>[4x]SNAMSEWSRI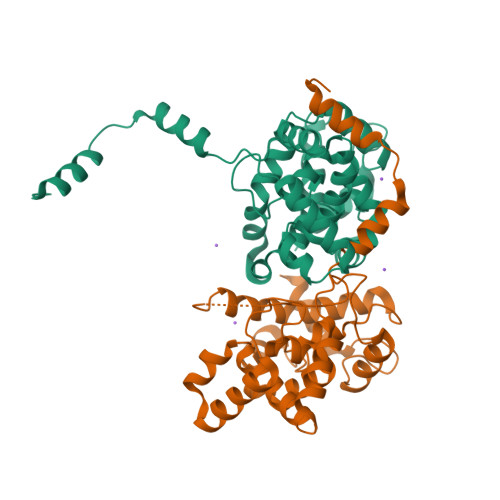AVEFGEQQLNLTELEDFARELAYEGLDPALIIKKLKETGGDDWVKDTKFIIVFALTDGNDIVKASGDMSNSGSKRLMALQEKYGLVERAETRLSITPVRVAQSLPTWTCAAAAALKEYLPVGPAVMNLKVENYPPEMMCMAFGSLIPTAGVSEATTKTLMEAYSLWQDAFTKTINVKMRGASKTEVYNSFRDPLHAAVNSVFFPNDVRVKWLKAKGILGPDGVPSRAAEVAAAAYRNL> PISADFSEVENAPSFLSLAENTDEVLKPYTGLEIQTIITNIVGDANPNQSRIFDQDRLRGNQYSAGGLVTQNAVSAIPFTNLIPRTIRVGNILVNSANRLQITETNVSEYYSNPIIATKLSEMISDQVKNNQFSTWRRDNTSLQGFNAFDIATINTAILPNGLSLESMLLKLSLLHSIKAMNVDAASINRSQYQVIDHNTVPTIGAPAVVGVNNSPVFGEDCGGNNPVYPFGGGTGAIAFHVTLQTVPDERKSYAIFVPPAILQATSDANEALALFALSMSEWPHALYTVTKQTTDLAGANAGQQVFIPTQSTIHIGGRRVLDLIIPRREIAPNPTTLVAANAMCMVRPQAGPDATAGAIPLAAGQLFNMNFIGAPAFEEWPLTSYLYSWAGRFDITTIRQYMGRLATMVGVKDAYWAAHELNVALSQVAPKMTTAAGGWAAQAANSAQQSDVCYSSLLTVTRSAANFPLANQPAADMRVYDTDPATWNKVALGLATAANLVPEQSMDVPFVVGDARTSFWERLQAIPMCIAWTMYYHSRGITTLAWDNAYTDNTNKWLQKMVRNTFSTTQSVGTIIPARYGKIVCNLYKNMFHRAPAYVATSVGGKELHITHFERWLPGGTYANVYSGAGAVVNCFSPVLIPDIWCQYFTAKLPLFAGAFPPAQGQNSTKGFNSKQGLMIHRNQNNNLVAPYLEKFADNSSYFPVGQGPEINDMATWNGRLWMTTGNVQYLDYSGAAIVEAVPPAGELPVGKQIPLLAGENAPIELTNAATTCVPRYSNDGRRIFTYLTTAQSVIPVQACNRAANLARSCWLLSNVYAEPALQALGDEVEDAFDTLTNS;> PISADFSEVENAPSFLSLAENTDEVLKPYTGLEIQTIITNIVGDANPNQSRIFDQDRLRGNQYSAGGLVTQNAVSAIPFTNLIPRTIRVGNILVNSANRLQITETNVSEYYSNPIIATKLSEMISDQVKNNQFSTWRRDNTSLQGFNAFDIATINTAILPNGLSLESMLLKLSLLHSIKAMNVDAASINRSQYQVIDHNTVPTIGAPAVVGVNNSPVFGEDCGGNNPVYPFGGGTGAIAFHVTL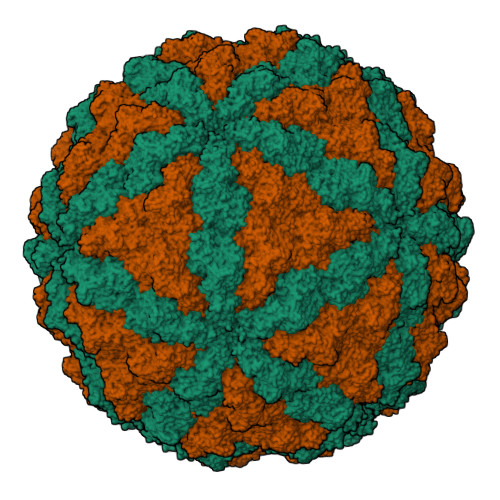QTVPDERKSYAIFVPPAILQATSDANEALALFALSMSEWPHALYTVTKQTTDLAGANAGQQVFIPTQSTIHIGGRRVLDLIIPRREIAPNPTTLVAANAMCMVRPQAGPDATAGAIPLAAGQLFNMNFIGAPAFEEWPLTSYLYSWAGRFDITTIRQYMGRLATMVGVKDAYWAAHELNVALSQVAPKMTTAAGGWAAQAANSAQQSDVCYSSLLTVTRSAANFPLANQPAADMRVYDTDPATWNKVALGLATAANLVPEQSMDVPFVVGDARTSFWERLQAIPMCIAWTMYYHSRGITTLAWDNAYTDNTNKWLQKMVRNTFSTTQSVGTIIPARYGKIVCNLYKNMFHRAPAYVATSVGGKELHITHFERWLPGGTYANVYSGAGAVVNCFSPVLIPDIWCQYFTAKLPLFAGAFPPAQGQNSTKGFNSKQGLMIHRNQNNNLVAPYLEKFADNSSYFPVGQGPEINDMATWNGRLWMTTGNVQYLDYSGAAIVEAVPPAGELPVGKQIPLLAGENAPIELTNAATTCVPRYSNDGRRIFTYLTTAQSVIPVQACNRAANLARSCWLLSNVYAEPALQALGDEVEDAFDTLTNSSF> GGGRGRLILEHTLQGHKGRIWGVAWHPKGNVFASCGEDKAIRIWSLTGNTWSTKTILSDGHKRTIREIRWSPCGQYLASASFDATTAIWSKSSGEFECNATLEGHENEVKSVSWSRSGGLLATCSRDKSVWIWEVAGDDEFECAAVLNPHTQDVKRVVWHPTKDILASASYDNTIKMFAEEPIDNDWDCTATLTSHTS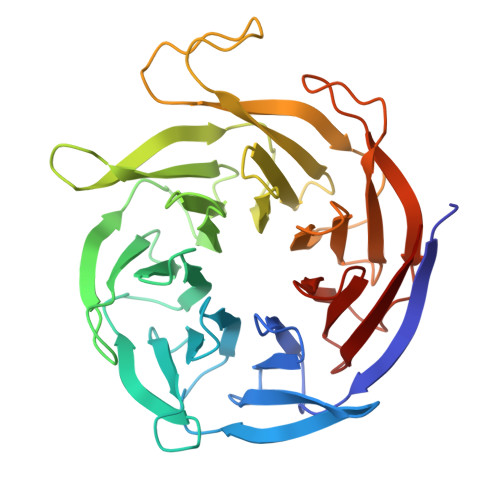TVWGIDFDADGERLVSCSDDTTIKIWRAYHPGNTAGVATPDQQTVWKCVCTVSGQHSRAIYDVSWCKLTGLIATACGDDGIRIFKESSDSKPDEPTFEQITAEEGAHDQDVNSVQWNPVVAGQLISCSDDGTIKIWKVTE> MGPLAFCGSENHSAAYRVDQGVLNNGCFVDALNVVPHVFLLFITFPILFIGWGSQSSKVHIHHSTWLHFPGHNLRWILTFMLLFVLVCEIAEGILSDGVTESHHLHLYMPAGMAFMAAVTSVVYYHNIETSNFPKLLIALLVYWTLAFITKTIKFVKFLDHAIGFSQLRFCLTGLLVILYGMLLLVEVNVIRVRRYIFFKTPREVKPPEDLQDLGVRFLQPFVNLLSKGTYWWMNAFIKTAHKKPIDLRAIGKLPIAMRALTNYQRLCEAFDAQVRKDIQGTQGARAIWQALSHAFGRRLVLSSTFRILADLLGFAGPLCIFGIVDHLGKENDVFQPKTQFLGVYFVSSQEFLANAYVLAVLLFLALLLQRTFLQASYYVAIETGINLRGAIQTKIYNKIMHLSTSNLSMGEMTAGQICNLVAIDTNQLMWFFFLCPNLWAMPVQIIVGVILLYYILGVSALIGAAVIILLAPVQYFVATKLSQAQRSTLEYSNERLKQTNEMLRGIKLLKLYAWENIFRTRVETTRRKEMTSLRAFAIYTSISIFMNTAIPIAAVLITFVGHVSFFKEADFSPSVAFASLSLFHILVTPLFLLSSVVRSTVKALVSVQKLSEFLSSAEIREEQCAPHEPTPQGPASKYQAVPLRVVNRKRPAREDCRGLTGPLQSLVPSADGDADNCCVQIMGGYFTWTPDGIPTLSNITIRIPRGQLTMIVGQVGCGKSSLLLAALGEMQKVSGAVFWSSLPDSEIGEDPSPERETATDLDIRKRGPVAYASQKPWLLNATVEENIIFESPFNKQRYKMVIEACSLQPDIDILPHGDQTQIGERGINLSGGQRQRISVARALYQHANVVFLDDPFSALDIHLSDHLMQAGILELLRDDKRTVVLVTHKLQYLPHADWIIAMKDGTIQREGTLKDFQRSECQLFEHWKTLMNRQDQELEKETVTERKATEPPQGLSRAMSSRDGLLQDEEEEEEEAAESEEDDNLSSMLHQRAEIPWRACAKYLSSAGILLLSLLVFSQLLKHMVLVAIDYWLAKWTDSALTLTPAARNCSLSQECTLDQTVYAMVFTVLCSLGIVLCLVTSVTVEWTGLKVAKRLHRSLLNRIILAPMRFFETTPLGSILNRFSSDCNTIDQHIPSTLECLSRSTLLCVSALAVISYVTPVFLVALLPLAIVCYFIQKYFRVASRDLQQLDDTTQLPLLSHFAETVEGLTTIRAFRYEARFQQKLLEYTDSNNIASLFLTAANRWLEVRMEYIGACVVLIAAVTSISNSLHRELSAGLVGLGLTYALMVSNYLNWMVRNLADMELQLGAVKRIHGLLKTEAESYEGLLAPSLIPKNWPDQGKIQIQNLSVRYDSSLKPVLKHVNALIAPGQKIGICGRTGSGKSSFSLAFFRMVDTFEGHIIIDGIDIAKLPLHTLRSRLSIILQDPVLFSGTIRFNLDPERKCSDSTLWEALEIAQLKLVVKALPGGLDAIITEGGENFSQGQRQLFCLARAFVRKTSIFIMDEATASIDM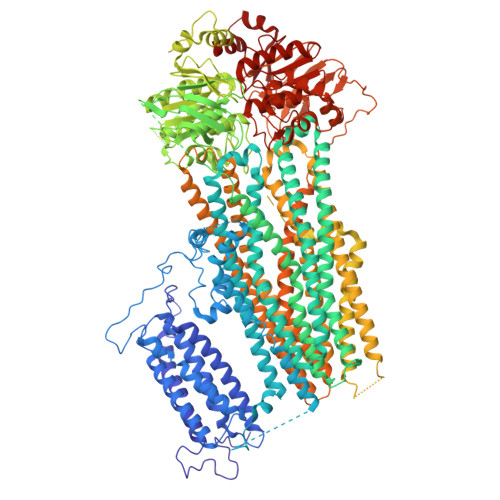ATENILQKVVMTAFADRTVVTIAHRVHTILSADLVIVLKRGAILEFDKPEKLLSRKDSVFASFVRADK>GPAVPRTGPDVSALQLLSNSFESVFDSPDDFYSDAKLVLSDGREVSFHRCVLSA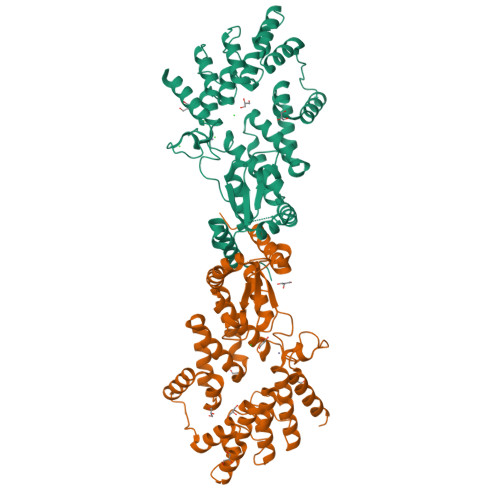RSSFFKSALAAAKKEKDSNNTAAVKLELKEIAKDYEVGFDSVVTVLAYVYSSRVRPPPKGVSECADENCCHVACRPAVDFMLEVLYLAFIFKIPELITLYQRHLLDVVDKVVIEDTLVILKLANICGKACMKLLDRCKEIIVKSNVDMVSLEKSLPEELVKEIIDRRKELGLEVPKVKKHVSNVHKALDSDDIELVKLLLKEDHTNLDDACALHFAVAYCNVKTATDLLKLDLADVNHRNPRGYTVLHVAAMRKEPQLILSLLEKGASASEATLEGRTALMIAKQATMAVECNNIPEQCKHSLKGRLCVEILEQEDKREQIPRDGGWSHPQFEK[2x]> MLRALWLFWILVAITVLFSKRCSAQESLSCDASGVCDGRSRSFTSIPSGLTAAMKSLDLSFNKITYIGHGDLRACANLQVLILKSSRINTIEGDAFYSLGSLEHLDLSDNHLSSLSSSWFGPLSSLKYLNLMGNPYQTLGVTSLFPNLTNLQTLRIGNVETFSEIRRIDFAGLTSLNELEIKALSLRNYQSQSLKSIRDIHHLTLHLSESAFLLEIFADILSSVRYLELRDTNLARFQFSPLPVDEVSSPMKKLAFRGSVLTDESFNELLKLLRYILELSEVEFDDCT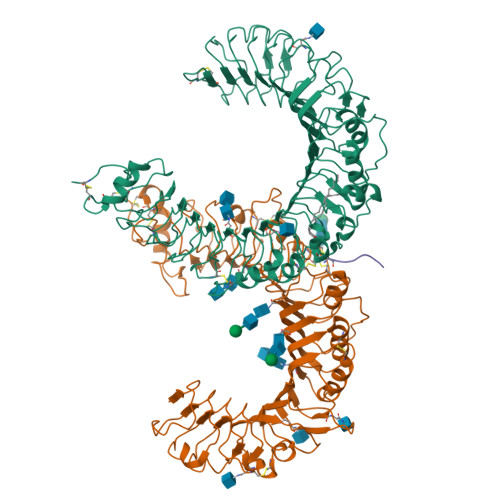LNGLGDFNPSESDVVSELGKVETVTIRRLHIPQFYLFYDLSTVYSLLEKVKRITVENSKVFLVPCSFSQHLKSLEFLDLSENLMVEEYLKNSACKGAWPSLQTLVLSQNHLRSMQKTGEILLTLKNLTSLDISRNTFHPMPDSCQWPEKMRFLNLSSTGIRVVKTCIPQTLEVLDVSNNNLDSFSLFLPRLQELYISRNKLKTLPDASLFPVLLVMKIASNQLKSVPDGIFDRLTSLQKIWLHTNPWDCSCPRIDYLSRWLNKNSQKEQGSAKCSGSGKPVRSIICPTLVPR;> MSQDRKPIVGSFHFVCALALIVGSMTPFSNELESMVDYSNRNLTHVPKDLPPRTKALSLSQNSISELRMPDISFLSELRVLRLSHNRIRSLDFHVFLFNQDLEYLDVSHNRLQNISCCPMASLRHLDLSFNDFDVLPVCKEFGNLTKLTFLGLSAAKFRQLDLLPVAHLHLSCILLDLVSYHIKGGETESLQIPNTTVLHLVFHPNSLFSVQVNMSVNALGHLQLSNIKLNDENCQRLMTFLSELTRGPTLLNVTLQHIETTWKCSVKLFQFFWPRPVEYLNIYNLTITERIDREEFTYSETALKSLMIEHVKNQVFLFSKEALYSVFAEMNIKMLSISDTPFIHMVCPPSPSSFTFLNFTQNVFTDSVFQGCSTLKRLQTLILQRNGLKNFFKVALMTKNMSSLETLDVSLNSLNSHAYDRTCAWAESILVLNLSSNMLTGSVFRCLPPKVKVLDLHNNRIMSIPKDVTHLQALQELNVASNQLKSVPDGVFDRLTSLQYIWLHDNPWDCTCPGIRYLSEWINKHSGVVRNSAGSVAPDSAKCSGSGKPVRSIICPTLVPR;> CSKKKK However, owing to genetic redundancy of the ABA receptors, how the ABA signal is perceived and transduced has been debated for a long time until a breakthrough in 2009 when a novel family of proteins containing steroidogenic acute regulatory protein (StAR)-related lipid-transfer (START) domain was discovered as ABA receptors. ABA-induced interaction of PYLs with PP2Cs releases the inhibitory effect of PP2Cs on SnRK2 protein kinases, resulting in the activation of SnRK2s and phosphorylation of the downstream targets such as ABF transcription factors. In this study, we identified several candidate genes for ABA receptors in the turfgrass Festuca elata and Zoysia japonica, and then we confirmed that one of the candidate receptors, named FePYR1, functions as an ABA receptor through crystal structure and biochemical analyses. Furthermore, we found that expression of FePYR1 significantly enhances drought resistance in transgenic Arabidopsis.

We attempted to crystalize the three ABA receptor proteins, and found that only the FePYR1-ABA complex generated high-quality and diffractable crystals. The structure of FePYR1-ABA was solved by molecular replacement starting from a model of the Arabidopsis thaliana protein AtPYL2 with the statistics of the structure refinement shown in Table S1. The FePYR1-ABA complex crystal structure was determined at a resolution of 2.7 Å, and the overall structure revealed a receptor/ligand complex with 1:1 stoichiometry. The ABA-bound FePYR1 appeared as a trimeric form arranged about 120° from each other in an asymmetric unit of the P42212 space group. Although FePYR1 has the highest sequence identity with AtPYR1, FePYR1 displayed a monomeric form in solution which is different from the dimeric AtPYR1. The electron density map shows that ABA is tethered in the 428.0 Å3 of protein cavity with its hydrocarbon chain and cyclohexene ring fitting closely into the hydrophobic pocket of FePYR1. The terminal carboxylate of ABA is anchored in the bottom of the cavity of FePYR1 by an interaction between the positively charged inward-pointing K72 side chain with the negatively charged carboxyl group of ABA. Based on the structural statistics of FePYR1-ABA and published data, E160 and N186 are assumed to form water-mediated hydrogen bonds with the acid head group of ABA. Figure 3B shows that the mono-methyl group on the cyclohexene ring fits into a narrow hydrophobic pocket formed by residues F74, I75, V100, L104, F178, and V182, while the dimethyl group fits into a larger pocket formed by A106, S109, I127 and H132. At top orientation of the cavity, the carbonyl group on the cyclohexene ring of ABA points to the cavity entrance and is capped by the P105 in the loop (β3–β4) as a gate, and the R133 in the loop (β5–β6) points across the entry as a latch.

>[3x]MEQQPAAAEPEVPAGLGLTAAEYAELQPTVEAYHRYAVGPGQCSSLVAQRIEAPAAAVWAIVRRFDCPQVYKHFIRSCALRPDPDAGDELRPGRLREVSVISGLPASTSTERLDLLDDARRAFGFTITGGEHRLANYRSVTTVSELAPAAPAKICTVVLESYVVDVPEGNSEEDTRLFADTVVRLNLQKLKSLAEANATSAAAQATPPPQAE> MEDGAQMRVVAFGDQTYDCSEAVSQLLRVRDDAIVVDFLERAPAVLKAELARLSSEQQEETPRFATLAELVPRYRAGTLNPAVSQALTCIAQLGLFIRQHSSGQEAYPTAHDSCITGVCTGALTAVAVGSASSVTALVPLALHTVAVAVRLGARAWEIGSCLADARRGANGRYASWTSAVGGISPQDLQDRISAYTAEQALASVSVPYLSAAVGPGQSSVSAAPVILDAFLSTLLRPLTTTRLPITAPYHAPHLFTAKDVQHVTDCLPPSEAWPTVRIPIISFSRDEAVSRGASFPAAMSEAVRDCLIRPIALDRMAVSIANHARDLGKDSVLPSPIALSFSDKLGPQVNSHLPGAKAPTPELTSKSIPSAIGAEQQPMAKSPIAILAASGRFPQSSSMDQFWDVLINGVDTHELVPPTRWNAATHVSEDPKAKNVSGTGFGCWLHEAGEFDAAYFNMSPREAPQVDPAQRLALLTATEALEQAGVVPNRTSSTQKNRVGVWYGATSNDWMETNSAQNVDTYFIPGGNRAFIPGRVNYFHKFSGPSYTIDTACSSSLAALHMACNALWRGEVDTAIVGGTNVLTNPDMTAGLDAGHFLSRSGNCKTFDDEADGYCRGEAVVTLILKRLPDAQADKDPIQASILGIATNHSAEAASITRPHAGAQQDLFQQVLTETGLTANDISVCEMAGTGTQAGDSGETTSVVETLAPLNRSGSAVRTTPLYIGAVKSNVGHAESAAGVSSLAKILLMLKHSKIPPHVGIKTKLNHRLPDLAARNTHIARSEVPWPRPKNGKRRVLLNNFSAAGGNTCLVLEDAPEPEDSQEVDPREHHIVALSAKTPDSMVNNLTNMITWIDKHSGDSLATLPQLSYTTTARRVHHRHRAVATGTDLLQIRSSLQEQLDRRVSGERSIPHPPNGPSFVLAFTGQGSAFAGMGVDLYKRFASFRSDIARYDQICEGMSLPSIKAMFEDEKVFSTASPTLQQLTHVCFQMALYRLWKSLGVQAKAVVGHALGEYAALYAAGVLSQSDTLYLVGRRAQLMEKHLSQGTHAMLAVRAKEEAIVAAIDGPPGEAYEFSCRNGEQRNVLGGTVAQIQAAK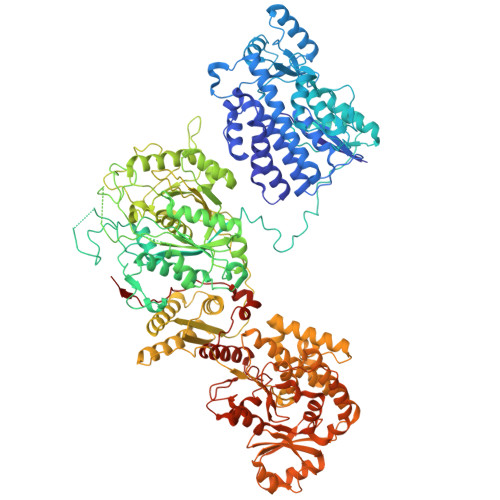AALEAKKIRCQYLDTPMAFHTGQVDPILPELLQVAAACSIQDPQIPVISPAYGKVIRSAKDFQPEYFTHHCRSSVNMVDALQSAVEEGLLDKNVIGLEIGPGPVVTQFVKEAVGTTMQTFASINKDKDTWQLMTQALAKFYLAGASVEWSRYHEDFPGAQKVLELPAYGWALKNYWLQYVNDWSLRKGDPAVVVAASAAALEHHHHHH(7S)-2-(3,5-difluoro-4-hydroxyanilino)-7-methyl-5-[(1,2-oxazol-5-yl)methyl]-8-(prop-2-yn-1-yl)-7,8-dihydropteridin-6(5H)-one 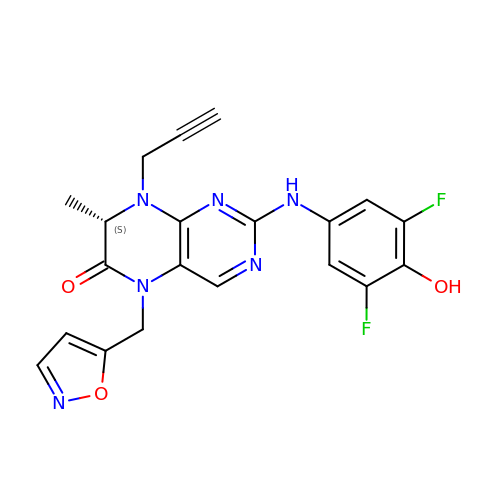| C20 H16 F2 N6 O3 | DFEBWFCZSQPYKA-NSHDSACASA-N Here, we report PET‐degrading α/β hydrolases, including HaloPETase1 from the marine Halopseudomonas lineage, thereby extending the narrow sequence space by novel features at the active site. The enzymatic degradation of polyethylene terephthalate (PET) offers a sustainable solution for PET recycling. HaloPETase1 is a salt‐tolerant enzyme and depends on higher salt concentrations for the degradation of PET at elevated temperatures. We propose an extension of this PETase classification system by type III PETases that include HaloPETase1, 2, 3, and 4, as well as PmC and dsPETase05.

The crystal structure of HaloPETase1 was determined to a resolution of 1.16 Å, revealing a unique active site architecture and a lack of the canonical π‐stacking clamp found in PETases so far. HaloPETase1 has the canonical α/β hydrolase fold illustrating highly conserved spatial positions for its catalytic residues S156, D206, and H236 as known for IsPETase (type IIb). There are two disulfide bonds observed: Db I (C64‐C126) and Db II (C273‐C276). While two bonds are characteristic for type II PETases, these are, however, located at different positions in HaloPETase1. Notably, we could not observe a disulfide bond flanking the active site, as it is known for IsPETase. In HaloPETase1, on the other hand, we observed the non‐conserved aromatic acid Y180 in subsite I (equivalent to W185 in IsPETase), which might form a π‐stacking interaction with the substrate. However, instead of an aromatic residue at the equivalent position of Y87 in IsPETase, we found T88 for HaloPETase1. Thus, the so‐called π‐stacking “clamp” does not exist for HaloPETase1. Further, we hypothesize that the backbone amide protons of T88 and Q157 are responsible for the formation of the oxyanion hole in HaloPETase1 since these residues are located at equivalent positions as M161 and Y87 in IsPETase. In contrast, HaloPETase1 has a distinct and extended loop (loop 3) due to an insertion of five amino acids.

> STNPGGGGGGSNPDTGTGFPGVSSFSADGSFATTSGSAGLSCTVFRPSTLGANGLKHPIIVWGNGTTASPSTYSGILEHWASHGFVVIAANTSNAGTGQDMLNCVDYLTTQNNRSTGTYANKLDLNRIGAAGHSQGGGGTIMAGQDYRIKVTAPFQPYTIGLGHNSSSQSNQNGPMFLMTGSADTIASPTLNALPVYNRANVPVFWGELSGASHFEPVGSAGDFRGPSTAWFRYHLMDDASAEDTFYGSNCDLCTDNDWEVRRKGINA> GPSQVIFNSVEKFYIPGGDVTCHYTFTQHFIPRRKDWIGIFRVGWKTTREYYTFMWVTLPIDLNNKSAKQQEVQFKAYYLPKDDEYYQFCYVDEDGVVRGASIPFQFRPENEEDILVVTTQGE

Autophagy receptors target cargo to autophagy by binding ATG8 on autophagosomal membranes. In this study we discovered that the ubiquitin-binding autophagy receptor NDP52 binds preferentially to LC3C, in contrast to other autophagy adaptors including p62 and NBR1 that nonselectively interact with several human ATG8 orthologs. NDP52 comprises an N-terminal SKICH domain of unknown structure (aa 1–127), a central coiled-coil forming region (aa 140–420) and a C-terminal ubiquitin-binding Zn finger domain (ZnF, aa 421–446). We determined the crystal structure of the NDP52 N terminus (aa 21–141) containing the SKICH domain and CLIR in isolation and in complex with LC3C.

Since the SKICH domain fold was unknown, experimental phasing was performed exploiting the anomalous scattering of cadmium ions contained in one of two independent crystal forms. Single anomalous dispersion (SAD) phasing of a 2.7 Å data set was used to build an initial model, which served in molecular replacement to determine the 1.35 Å crystal structure of the NDP52 SKICH domain in a different space group. The structure revealed a β sandwich fold comprising seven antiparallel β strands, organized in two sheets of four and three strands. Some loops connecting the seven β strands of NDP52 fold back to form hydrophobic interactions with the β sheets. The SKICH domain resembles an Ig-fold lacking the eighth β strand, which places the N and C termini onto opposite sides of the β sandwich. The specificity of NDP52 for LC3C is mediated by a noncanonical LIR comprising the tripeptide Leu-Val-Val, which we refer to as the CLIR motif. This binding site in NDP52, located between the SKICH domain and a coiled-coil forming region, is distinct from a previously predicted LIR within the SKICH domain, i.e., Trp-Ile-Gly-Ile55-58 (Kraft et al., 2010). While this sequence is reminiscent of a LIR motif, our structure reveals it to be buried in a β sandwich-fold and inaccessible for canonical ATG8 interactions.>[2x]MRVTQKLNHGWIFAEGAADPATPLAGETVTLPHNAVDLPLSYFDETSYQRAFTYQRVIAWDDAWQGRRVQLRFDGAMADNVVWVNGVQVVAHPDGYTPFVADLTDHLRPGDNLVTVRIDGSENPAIPPFGAQIDYLTYAGIYRDVWLMVLPERHLTNARILTPDALSDAKTVVIRPEVTAPGPVRARLLDGD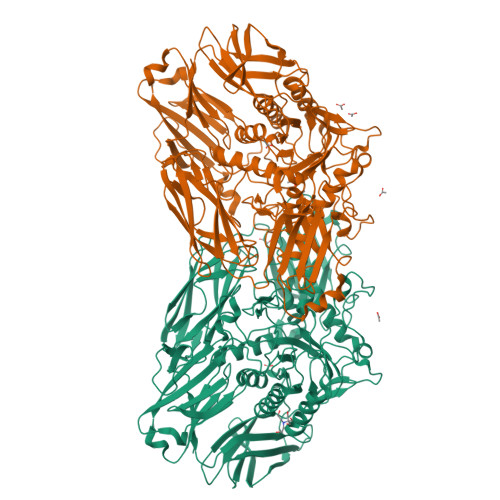REIAATEGEGELTLAGLTGLSLWSTDNPQLYTVELTLPDSGDVTTHRFGFRTAEWTPQGFLLNGQPMKLRGLNRHQSWAHQGYAAGRHAQERDAEIVRHDLCCNMVRTSHYPQSTWFLDRCDEIGLLVFEEIPGWQHIGDQAWQDRSVDNVRAMITRDWNHPSIVIWGVRINESPDNHDFYVRTNALARELDPTRAIGGVRCITDSEMLEDVYTMNDFILDESELPLINRPRTALRPTEEVTGIKKPVPYLVTEYNGHMFPTKAQDPELRQMEHVIRHLEVLNAAHGDPAISGCIGWCMFDYNTHKDFGAGDRICHHGVMDIWREPKFAAHAYGSQKPPSEGIVMEPVTFWARGERNIGGVLPLIVLTNCDEVEFECAGVTRRVGPDRERFPHLPRPPVIIDHRHISAEELGQWGMSWHPGRITGWLNGEQVALREYVADPLPTTLQIAPDRDTLPADGDIDLRVMLRALDQVGNRLPFLDAGIAVTVDGPARLIGPDLRMLQGGTTGMLLRLTGDAGTIRITARHPQFPEAVATVTVG> DRAPEGNYVDATFYTSDEALEAATAPLYNRAWFDYNQRSIVPIGSGRANDMYSPWNYPQFVTFQVTALDENLSGAWSGFYSVVTMANSVINAVETQTQGSVSEAAKTKAIAEARLMRACA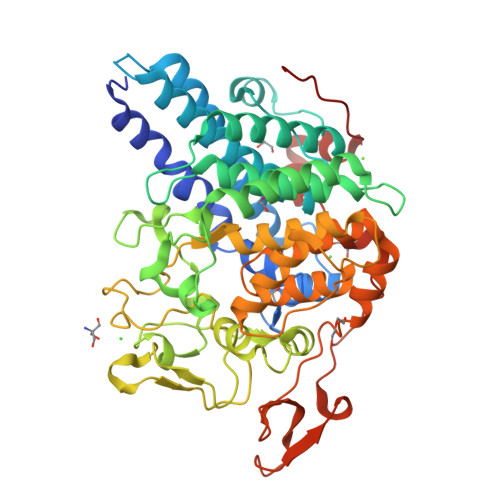YFYMLRIWGPVILIEDNQKLVDNPVRPLNREEDVFQFIINDLNYAVDNLSEQSDKGRATSWAAKGILAKVYLARSGWNNGGTRDEGDLELARQYASDVCENSGLDLMTNYEDLFKYKNNNNQESLLAMQWVPLGEWYECNTLLSDLAFSTEVTGGVNCWSSYNGSIDMLQQYELADTLRRNATFFTKGSYYSYICIKDGGYTYKGTASPIKKGVPGGPDDDNDGKVKQMNSPLNTYILRLADVYLTYAEACLGNNSTLSDGRGLYFFNRVRERAKINKKSSITLDDIIRERRVEFGMEYSNWYDMVTWFRYLPDKMLNYFNNQWRGYRTDAIIKDEDGKLHFGKYDTDGTTFLEGPEYYTAPEFTINIEAEDIFLPYPESDVIQNPLLNEPPVPYTFNE> GPAMAHMNSMDRHIQQTNDRLQCIKQHLQNPANFHNAATELLDWCGDP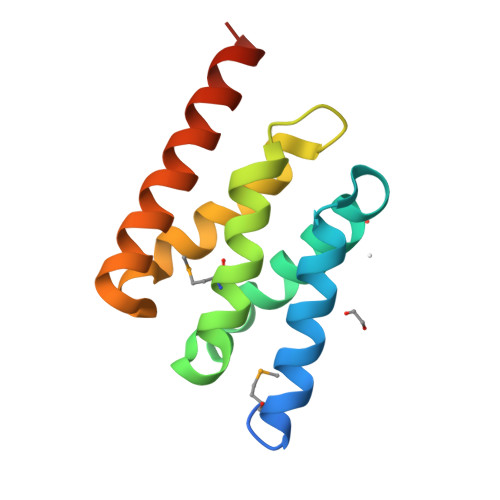RAFQRPFEQSLMGCLTVVSRVAAQQGFDLDLGYRLLAVCAANRDKFTPKSAALLSSWCEELGRLLLLRHQKSRQSD> CGAEPPAEEHVRVLAQTVKMAEFASATSITGDIQARVQADQSFRVGGKIVERLVDVGDHVAAGQVLARLDPQDQRSNVENAQAAVAAQQAQSKLADLNYQRQKALLPKGYTSQSEYDQALASVRSAQSSLKAAQAQLANARDLLSYTE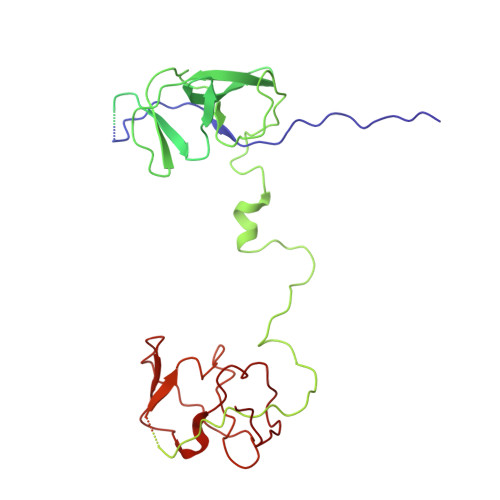LRASDAGVITARQAEVGQVVQATVPIFTLARDGERDAVFNVYESLFSHDVDGQRITVSLLGKPEVTASGKVREITPTVDERSGTLKVKVGLDSVPAEMSLGSVVNASVAAPAEHSVVLPWSALSKVGEQPAVWLLDQQGKARLQPVRVARYASEKVVIDGGLEAGQTVVTVGGQLLHPGQVVEVAQPPQPTQSTASRDAVGGGQPGNSRGGDEPPPAPPRPVLTVTVKTLKNDDLGRFAGSIQARYESVLGFRTNGRIASRLFDVGDFVGKGALLATLDPTDQQNQLRASQGDLASAEAQLIDAQANARRQEELFARSVTAQARLDDARTRLKTSQASFDQAKAAVQQARDQLSYTRLVTDFDGVITTWHAEAGQVVSAGQAVVTLARPEVREAVFDLPTEVAESLPADARFLVSAQLDPQARTTGSIRELGPQADASTRTRRVRLSLAQTPEAFRLGSTIQVQLSSAGSVRSVLPASVLLERDGKTQVWVVDGKQSSVALREVQVLSRDERQVVIGQGLADGDRVVRAGVNSLKPGQKIKLDEDAR> EDTVGRPLPHLAAAMQASGEAVYCDDIPRYENELFLRLVTSTRAHAKIKSIDVSEAQKVPGFVCFLSADDIPGSNETGLFNDETVFAKDTVTCVGHIIGAVVADTPEHAERAAHVVKVTYEDLPAIITIEDAIKNNSFYGSELKIEKGDLKKGFSEADNVVSGELYIGGQDHFYLETHCTIAIPKGEEGEMELFVSTQNAMKTQSFVAKMLGVPVNRILVRVKRMGGGFGGKETRSTLVSVAVALAAYKTGHPVRCMLDRNEDMLITGGRHPFLARYKVGFMKTGTIVALEVDHYSNAGNSRDLSHSIMERALFHMDNCYKIPNIRGTGRLCKTNLSSNTAFRGFGGPQALFIAENWMSEVAVTCGLPAE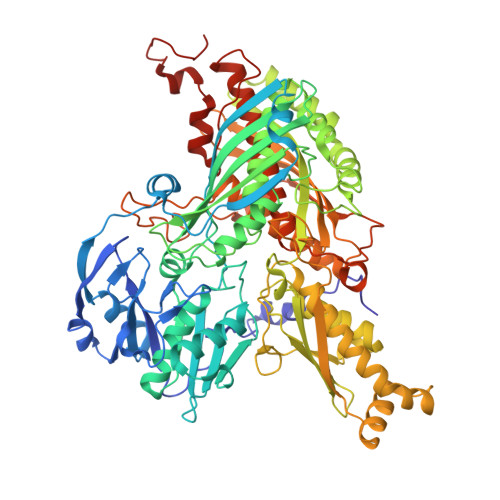EVRWKNMYKEGDLTHFNQRLEGFSVPRCWDECLKSSQYYARKSEVDKFNKENCWKKRGLCIIPTKFGISFTVPFLNQAGALIHVYTDGSVLVSHGGTEMGQGLHTKMVQVASKALKIPISKIYISETSTNTVPNSSPTAASVSTDIYGQAVYEACQTILKRLEPFKKKNPDGSWEDWVMAAYQDRVSLSTTGFYRTPNLGYSFETNSGNAFHYFTYGVACSEVEIDCLTGDHKNLRTDIVMDVGSSLNPAIDIGQVEGAFVQGLGLFTLEELHYSPEGSLHTRGPSTYKIPAFGSIPTEFRVSLLRDCPNKKAIYASKAVGEPPLFLGASVFFAIKDAIRAARAQHTNNNTKELFRLDSPATPEKIRNACVDKFTTLCVTGAPGNCKPWSLRV>[6x]MATPHINAEMGDFADVVL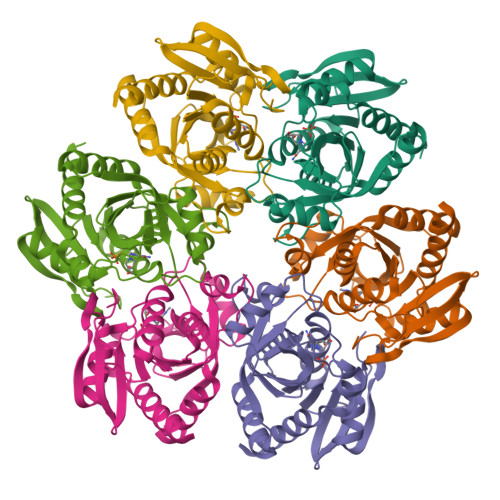MPGDPLRAKFIAETFLQDVREVNNVRGMLGFTGTYKGRKISVMGHGMGIPSCSIYAKELITDFGVKKIIRVGSCGAVRTDVKLRDVVIGMGACTDSKVNRMRFKDHDYAAIADFEMTRNAVDAAKAKGVNVRVGNLFSADLFYTPDPQMFDVMEKYGILGVEMEAAGIYGVAAEFGAKALTICTVSDHIRTGEQTTAAERQTTFNDMIEIALESVLLGDNA1-[(3~{R})-3-(4-azanylpyrazolo[3,4-d]pyrimidin-1-yl)piperidin-1-yl]propan-1-one | C13 H18 N6 O | 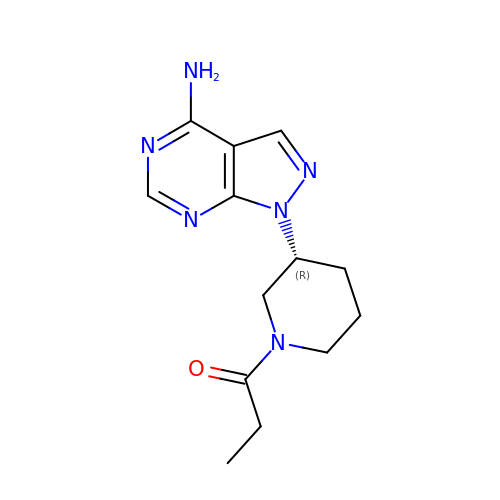VODQVZMDWITJDU-SECBINFHSA-N N-((1R,3R)-3-(7-(4-fluoro-2-methoxyphenyl)-3H-imidazo[4,5-b]pyridin-2-yl)cyclopentyl)acetamide | C20 H21 F N4 O2 | 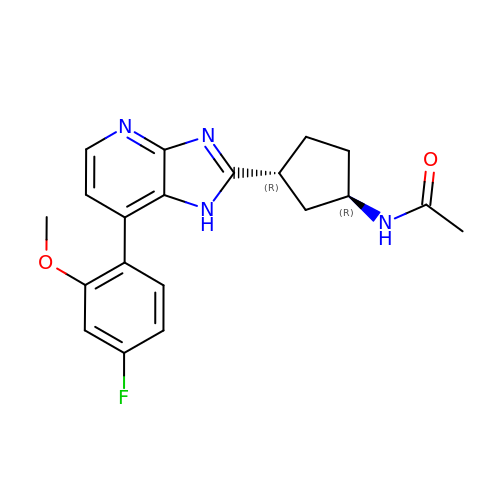KPPLCUYUCVJBTH-TZMCWYRMSA-N>MSNPTKISILGRESIIADFGLWRNYVAKDLISDCSSTTYVLVTDTNIGSIYTPSFEEAFRKRAAEITPSPRLLIYNRPPGEVSKSRQTKADIEDWMLSQNPPCGRDTVVIALGGGVIGDLTGFVASTYMRGVRYVQVPTTLLAMVDSSIGGKTAIDTPLG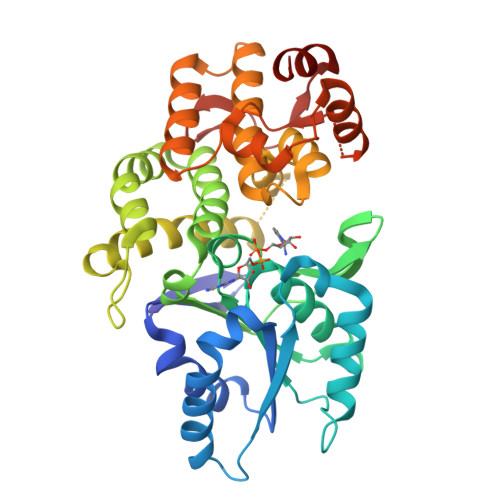KNLIGAIWQPTKIYIDLEFLETLPVREFINGMAEVIKTAAISSEEEFTALEENAETILKAVRREVTPGEHRFEGTEEILKARILASARHKAYVVSADEREGGLRNLLNWGHSIGHAIEAILTPQILHGECVAIGMVKEAELARHLGILKGVAVSRIVKCLAAYGLPTSLKDARIRKLTAGKHCSVDQLMFNMALDKKNDGPKKKIVLLSAIGTPYETRASVVANEDIRVVLAP[2x]>[7x]MVIPYVIEQTARGERVYDIYSRLLKDRIIFLGTPIDAQVANVVVAQLLFLDAQNPNQEIKLYINSPGGEVDAGLAIYDTMQFVRAPVSTIVIGMAASMA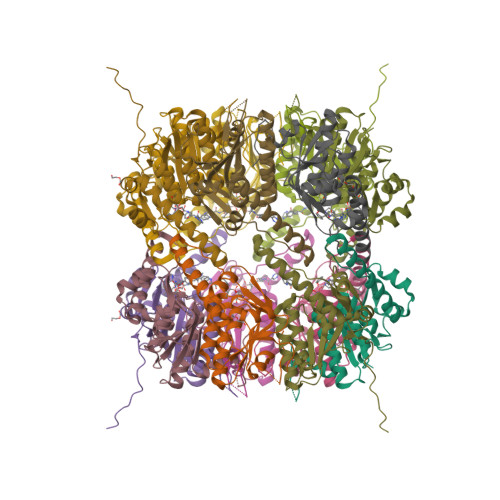AVILAAGEKGRRYALPHAKVMIHQPWGGVRGTASDIAIQAQEILKAKKLLNEILAKHTGQPLEKVEKDTDRDYYLSAQEALEYGLIDQVVTREEALEHHHHHHHH>MSSRVSTRSSLAEDLRAIGLADGDAVLVHAALRKVGKIVGGPDDILDAMRDVIGPAGTVLGYADWQLEDEIRDDPAMREHIPAFDPLRSRSIRDNGFWPELIRTTPGALRSASPGASMAAIGGEAEWFTADHALDYGYGPRSPLGKLVEAKGKVLMLGAPLDTMTLLHHAEHLADFPNKRILRYEAPILVDGEKVWRWFEEFDTSDPPDGLADDYFAGIVEEFLATGRGKRGKIGEASSVLVPADEIVAFAVDWLERWGRTAR[6x]

Here, we conduct a comprehensive functional analysis of the Antibiotic_NAT family of aminoglycoside acetyltransferases. AG resistance is primarily conferred by three classes of aminoglycoside-modifying enzymes (AMEs): phosphotransferases (APHs), nucleotidylyltransferases (ANTs), and acetyltransferases (AACs). AMEs permanently alter the AG substrate, preventing them from binding to their target, the A-site of the 16S rRNA in the bacterial ribosome. The fold typical of the Antibiotic_NAT family is evident in all structures, composed of 13 α-helices and 8 β-strands, and determined structures superpose with pairwise RMSD’s 0.8–1.0 Å between 197 to 266 matching Cα atoms.

Our data presented above demonstrated that the environmental metagenome-derived meta-AAC0038 enzyme can confer high and broad resistance to AGs including to the atypical AG apramycin when expressed in E. coli. Group 3 enzymes including AAC(3)-IIIb and four meta-AACs confer resistance to 4,6- and 4,5-disubstituted AGs, consistent with previous data reported for AAC(3)-III enzymes; meta-AAC0038 is the lone member of this family that confers resistance to apramycin. The meta-AAC0038 adopts a dimeric structure with a buried surface of ~900 Å2 per subunit. This enzyme also forms a dimer in solution according to the size exclusion chromatography (not shown). Similar sequence signatures (residues Thr165-Glu171 in meta-AAC0038) were identified in all analyzed members of this family, with His and Glu (His168 and Glu171 in meta-AAC0038) along with two glycine residues (Gly122 and Gly158 in metaAAC0038), completely conserved. The meta-AAC0038 and AAC(3)-IIIb structures superimpose with RMSD 0.54 Å across 219 Cα atoms, share all the minor subdomain structural elements, and show complete conservation of AG binding residues. However, the position corresponding to Glu223 in AAC(3)-IIIb is occupied by Asp213 in meta-AAC0038.>AEAGITGTWYNQLGSTFIVTAGADGALTGTYESAVGNAESRYVLTGRYDSAPATDGSGTALGWTVAWKNNYRNAHSATTWSGQYVGGAEARINTQWLLTSGTTEANAWKSTLVGHDTFTKV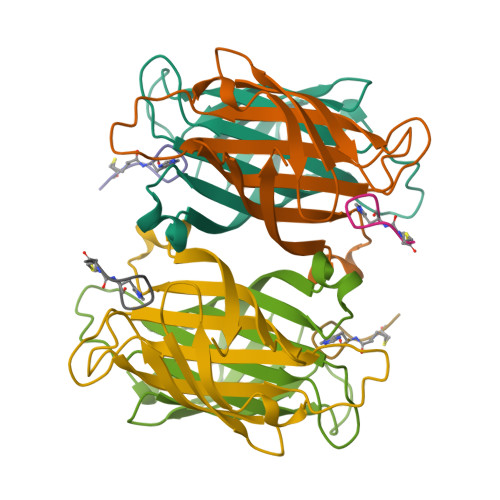KP[2x];>HPQGPPCKX[2x]>ANFLAMVDNLQGDSGRGYYLEMLIGTPPQKLQILVDTGSSNFAVAGTPHSYIDTYFDTERSSTYRSKGFDVTVKYTQGSWTGFVGEDLVTIPKGFNTSFLVNIATIFESENFFLPGIKWNGILGLAYATLAKPSSSLETFFDSLVTQANIPNVFSMQMCGAGLPVAGSGTNGGSLVLGGIEPSLYKGDIWYTPIKEEWYYQIEILKLEIGGQSLNLDCREYNADKAIVDSGTTLLRLPQKVFDAVVEAVARASLIPAFSDGFWTGSQL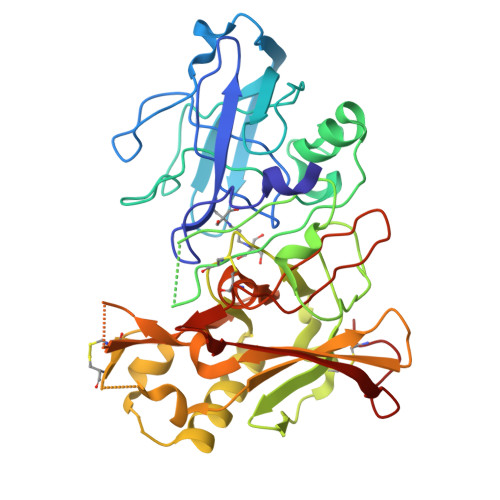ACWTNSETPWSYFPKISIYLRDENSSRSFRITILPQLYIQPMMGAGLNYECYRFGISPSTNALVIGATVMEGFYVIFDRAQKRVGFAASPCAEIAGAAVSEISGPFSTEDVASNCVPA[2x]>[2x]NEQRMGRKLAATTLKQCLAKGGARTAFPGTSEYSTARLAYNLRERYAPSAFVFPTTVAQVQNAVFCAKQVGVGIVPRGGGHSYEDYSLGGRDGVLVVDMEGFKQFSYNKAAKTAVVGAGFRLGPLYLA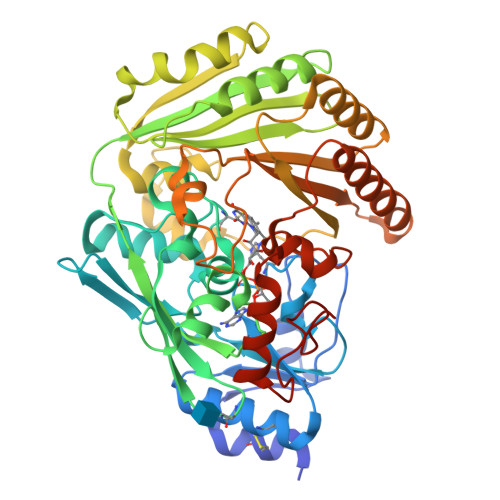LWNAGKVTIPAGNCPTVGIAGHALGGGWGFSSRKFGLVTDNILEVQLVAANGTVVTANAQKNKDLYFAIRGAGATSYGIVTQFTFRVHDVSAPVTHFKYRWNDKAVLFKNFKSFQSWGLNVPAEISAAFYMDPSGVSWLEGTYLGKKTSLLPLVKTFLASAAPNPTRVEEELNWIQLILVNWNYPSNTNPNQLNNVPFTTNTFKAKSIYVNGPGLSDAGINAMINAMNTGSNAYFIYDLYGSQSAINKVVPGETAFIHRNSLYSIQMVASWSNDNNAVTQTSYITRYWKVVRTYATGQAYQNYIDRDMPLSAYYGSSLSTLIAGKKKWDPQNVFNFPQSIPLKHHHHHHHH>STEKTVDQPKEDTHAIYKVENRHDYGTKGTKVDILTNHILLAVGNDVPTEKIDKELVPKLDGWWKTAFIFTYHIDFKPQQKGPPRRGKPVPPQELSKPKKYELIEALLDEDEILYKYRDRIAFNGEDTIYSHVPLEEFTLFDGCWEVSNKQKKKVVPGMGAPSNKASLQKKIDPELEEMVSQITLKFSGKVGLKDIYNDTTTQDTEVQESRMSAIDKTCLLSLLGAKFMSTDDLIFQVQGNKFFIFNNFAKAIPFQIGGYLLQGFTVSLTHVYGGVALNTVSVPAPFIKHTKYLPGDPRFKNNEKEQFTLMDWIIECYHQSKAIRDIRYNPKTAPPPSVKDLNYFVEKNTDISALLKGLKVYRPYINYSINKDGTPKPPRKRSSKGIVGFTRESAVSMRFNVLESSLKKNSAPKPNEKPININTIDYFKRKYDITLKYPDMKLVNLGGKNDVVPPECLTIVPGQKLKGQIFDTKTYIDFSAIRPTEKFDLISRLSMPAIKRGLTDSEKEESSAPH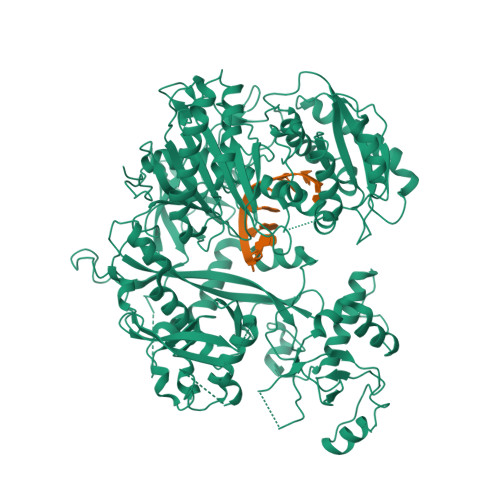NSAYQFMRVPSRILDAPVVQFKESTFEYKDKSYGTKHEESKGNWNMKGHQFISTPAKQVNLRAIFINNANTAPPASMESELDISMDKFASDVKQLGVDFNVSGKPILINQFGPPIKKFQGGGRGGRGGRGSRGGRGGRGAPSGPPTFETSPGEISLLNLLENIPSNTYILYVLRRGNDSAVYDRLKYITDLKFGALNSCVVWDNFKKNSIQYNSNVVMKMNLKLLGSNHSLSIENNKLLIDKESNLPILVLGSDVTHYPEKDQNSIASLVGSYDDKFTQFPGDYMLQDGPGEEIITNVGSLMLNRLKIYQKHNNGKLPTKIMYFRDGVSVDQFSQVVKIEVKSIKESVRKFGPQLNGGNKYDPPVTCIATVKRNQVRFIPIQENAKNEKGEEVAVQSMGNVMPGTVVDRGITSVAHFDFFIQSHQALKGTGVPCHYWCLYDENQSTSDYLQEICNNLCYIFGRSTTSVKVPAPVYYADLLCTRATCFFKAGFELNMAQAPKEKGSKDQPTVSKNVLLPQVNDNIKSVMYYI[2x]> AHMAHAGRSGYDNREIVMKYIHY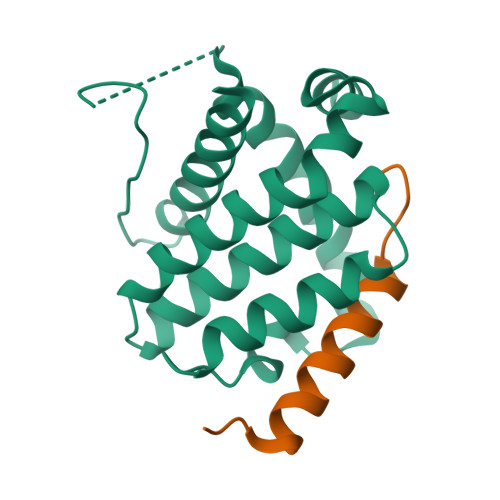KLSQRGYEWDAGDDAEENRTEAPEGTESEVVHLALRQAGDDFSRRYRRDFAEMSSQLHLTPFTARGCFATVVEELFRDGVNWGRIVAFFEFGGVMCVESVNREMSPLVDNIALWMTEYLNRHLHTWIQDNGGWDAFVELYGPSMR;> EYIKDCVFKDWEELGEEIRLKVFVLG> MQFLNMFFFDIYPYIAGAVFLIGSWLRYDYGQYTWRAASSQMLDRKGMNLASNLFHIGILGIFVGHFFGMLTPHWMYEAWLPIEVAQKMAMFAGGASGVLCLIGGVLLLKRRLFSPRVRATTTGADILILSLLVIQCALGLLTIPFSAQHMDGSEMMKLVGWAQSVVTFHGGASQHLDGVAFIFRLHLVLGMTLFLLFPFSRLI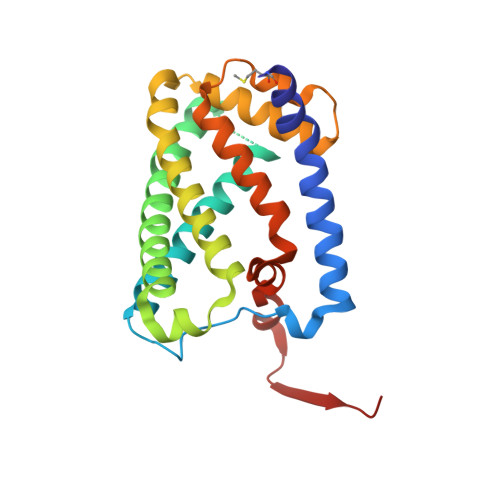HIWSVPVEYLTRKYQLVRARH> MKFAEHLSAHITPEWRKQYIQYEAFKDMLYSAQDQAPSVEVTDEDTVKRYFAKFEEKFFQTCEKELAKINTFYSEKLAEAQRRFATLQNELQSSLDAQKESTGVTTLRQRRKPVFHLSHEERVQHRNIKDLKLAFSEFYLSLILLQNYQNLNFTGFRKILKKHDKILETSRGADWRVAHVEVAPFYTCKKINQLISETEAVVTNELEDGDRQKAMKRLRVPPLGAAQPAPAWTTFRVGLFCGIFIVLNITLVLAAVFKLETDRSIWPLIRIYRGGFLLIEFLFLLGINTYGWRQAGVNHVLIFELNPRSNLSHQHLFEIAGFLGILWCLSLLACFFAPISVIPTYVYPLALYGFMVFFLINPTKTFYYKSRFWLLKLLFRVFTAPFHKVGFADFWLADQLNSLSVILMDLEYMICFYSLELKWDESKGLLPNNSEESGICHKYTYGVRAIVQCIPAWLRFI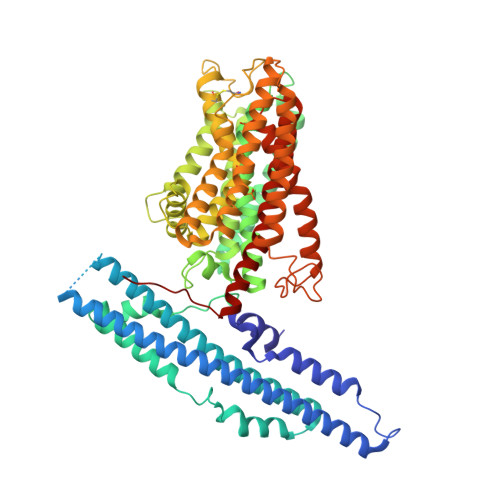QCLRRYRDTKRAFPHLVNAGKYSTTFFMVTFAALYSTHKERGHSDTMVFFYLWIVFYIISSCYTLIWDLKMDWGLFDKNAGENTFLREEIVYPQKAYYYCAIIEDVILRFAWTIQISITSTTLLPHSGDIIATVFAPLEVFRRFVWNFFRLENEHLNNCGEFRAVRDISVA>[2x]PSVYDAAAQLTADVKK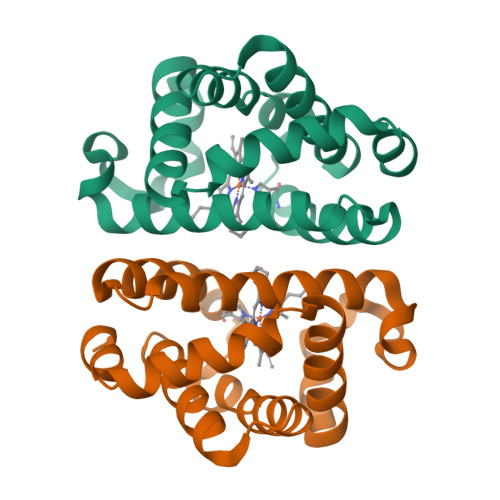DLRDSWKVIGSDKKGNGVALMTTLFADNQETIGYFKRLGDVSQGMANDKLRGHSITLMYALQNFIDQLDNPDDLVCVVEKFAVAHITRKISAAEFGKINGPIKKVLASKNFGDKYANAWAKLVAVVQAAL> QDSTSDLIPAPPLSKVPLQQNFQDNQFHGKWYVVGRAGNTGLREDKDPGKMFATIYELKEDKSYNVTYVWFGQKKCMYSIGTFVPGSQPGEFTLGNIKSAPGRTSWLVRVVSTNYNQHAMVFFKSVTQNREGFAITLYGRTKELTSELK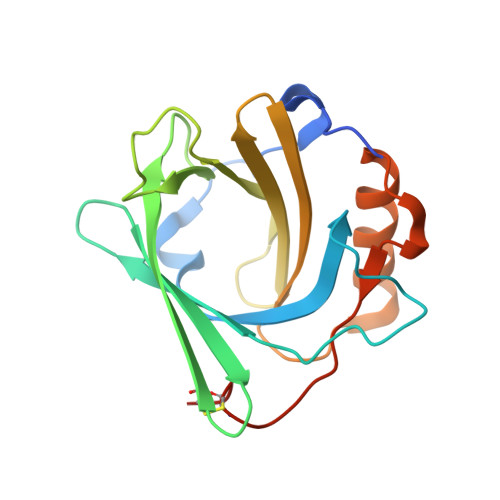ENFIRFSKSLGLPENHIVFPVPIDQCIDGSAHHHHHH> MQRQVIRRLGNRSAFPLV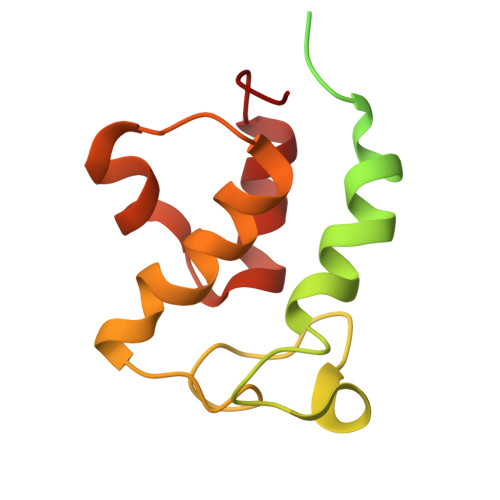AAVARSSQIRGAVRGDSGSRARVIPSFMCSLRAYSGGHHEEPSSRSGQYLLDKSDVLTRVLEVVKNFEKVDASKVTPESHFVKDLGLNSLDVVEVVFAIEQEFILDIPDHDAEKIQSIPDAVEYIAQNPMAK> MASPRAEQKQQTRHALMSAARHLMESGRGFGSLSLREVTRAAGIVPAGFYRHFSDMDQLGLALVAEVDETFRATLRAVRRNEFELGGLIDASVRIFLDAVGANRSQFLFLAREQYGGSLPIRQAIASLRQRITDDLAADLALLNKMPHLDGAALDVFADLVVKTVFATLPELIDPPAADLPPHLMPAAKITHQLRFIMIGGKHWHGLPGSSV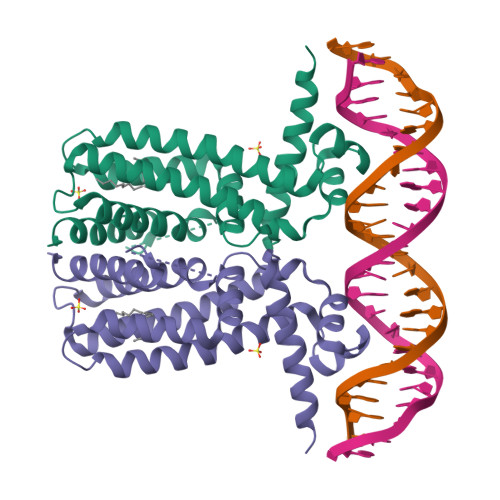DKLAAALE> GAMAMSDLPIEFTELVDLMSLGISPQFLDFRSTTFESDHFVTVRETKDGTNSVAIVDLAKGNEVTRKNMGGDSAIMHPSQMVISVRANGTIVQIFNLETKSKLKSFTLDEPVIFWRWLSETTLGFVTARSILTSNVFDGNVNAKPQLLTLRHANLNNTQIINFVANKNLDWFAVVGILQENGRIAGRIQLFSKQRNISQAIDGHVAIFTNILLEGNGSTPVQVFVTGNRNATTGAGELRIIEIDHDASLPSQYQKETTDIFFPPDATNDFPIAVQVSEKYGIIYLLTKYGFIHLYELETGTNLFVNRITAESVFTAAPYNHENGIACINKKGQVLAVEISTSQIVPYILNKLSNVALALIVATRGGLPGADDL;>GYTLIDL[3x]

The protein that gives the process its name, Clathrin, is a triskelion composed of three heavy chains (Clathrin Heavy Chain, Chc) that provide the structural backbone of the lattice, further stabilized and regulated by three light chains (Clathrin Light Chain, Clc). The proximal domain specifically interacts with Clcs, whereas, the N-terminal domain (NTD) of Chc, which adopts a WD40 beta-propeller structure, is pivotal for interactions with various adaptor proteins (APs). To investigate the existence of binding sites present in Clathrin NTD, we crystallized the N-terminal domain of Chc with different peptides derived from adaptor proteins containing CBMs. All our structures show that each peptide binds to three different binding pockets (Clathrin, Arrestin and W-box).

Crystal structure of Chc-NTD (displayed as a grey cartoon) bound to CBMs from Ent1 (1.75 Å, red), Ent2 (1.74 Å, yellow), Ent5 (Ent5.1 LIDL motif, 2.01 Å, green), Apl2.1 (Apl2.1 LLDLF motif, 2.75 Å, blue) and Yap1801 (1.95 Å, grey). For the Ent1 and Ent2 complexes, a water molecule bridges the interaction between the carbonyl oxygen at the motif’s +3 position and N64. Water-mediated interactions are also observed in the W-box between the NTD backbone (L24, D25 and V309) and the peptide at position +3, for both Ent1 and Ent2. Residue K284 within the W-box establishes salt bridges with the carboxy-terminal of Ent1, Ent2 and Yap1801. Mutation of the Clathrin box showed a reduction of almost seven-fold in the binding affinity to Ent1 (KDApp WT ≅ 138 µM vs. KDApp Cla ≅ 968 µM), while Ent2 exhibits a three-fold increase in its dissociation constant (KDApp Cla ≅ 509 µM). This data confirms Ent1’s binding preference towards the Clathrin box. Mutagenesis experiments conducted on clathrin binding sites revealed a consistent preference of Ent1 for the Clathrin box, with the Arrestin and W-boxes appearing to play a less critical role for Ent1, serving as secondary sites of interaction. Competition experiments conducted at sub saturating concentrations using native MS revealed that Ent1 is able to displace Ent2 but not vice versa. Here, we show that Ent1 binds more efficiently to Chc and therefore can be better recruited than Ent2.> GPHMREYKLVVLGSGGVGKSALTVQFVQGIFVEKYDPTIEDSYRKQVEVDAQQCMLEILDTAGTEQFTAMRDLYMKNGQGFALVYSITAQSTFNDLQDLREQILRVKDTDDVPMILVGNKCDLEDERVVGKEQGQNLARQWNNCAFLESSAKSKINVNEIFYDLVRQINSGGSGSGSSGGSGSGGGSG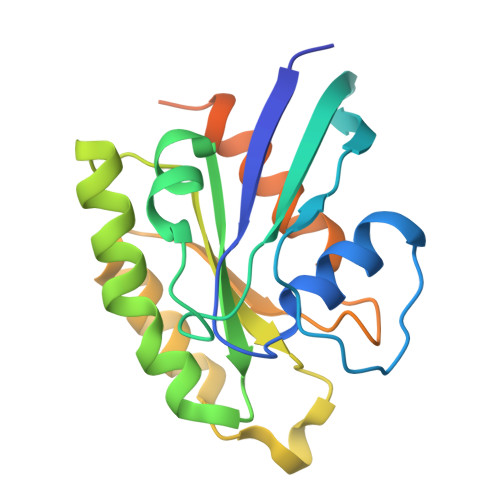SGSSGLPETGG>MVVKVGVIGTGAMGRAHIDRLTNVLTGAEVVAVTDIDHEAAEAAVRDFHLNAKVYPDDTSLLQDPDIDAVFVVSFGGAHEATVLKALDTDKFIFTEKPLATTLEGAKRIVDKELTKSKKVIQVGFMRRYDQGIRALKEKLDTGIIGAPLVVRASHINPNVASNYSNEMAITDTLIHEIDEMHWLLDDEYTSIQITYPRQSAEVRNEGLHDPQLATLTTKKGTVIQVLVHVTAQYGYEVKLEVIGETGELQLPNYGLGPILRSNANQQTAVEMSWINRFIQAYNTEVQEFIDEVAKSEPPVGPSAWDGYIAAITAAAANRSQKDQETVLINVAGT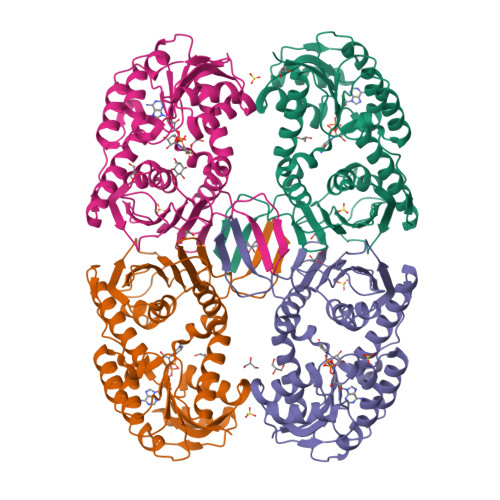PTFYQ[4x]>MGSSHHHHHHHHHHSSGLVPRGSGGSMSAIGTVFKEHVKNFYLIQRLAQFQVKIINHSNYLGVAWELINPVMQIMVYWMVFGLGIRSNAPIHGVPFVYWLLVGISMWFFINQGILEGTKAITQKFNQVSKMNFPLSIIPTYIVTSRFYGHLGLLLLVIIACMFTGIYPSIHIIQLLIYVPFCFFLTASVTLLTSTLGVLVRDTQMLMQAILRILFYFSPILWLPKNHGISGLIHEMMKYNPVYFIAESYRAAILYHEWYFMDHWKLMLYNFGIVAIFFAIGAYLHMKYRDQFADFL[2x];>MNVSVNIKNVTKEYRIYRTNKERMKDALIPKHKNKTFFALDDISLKAYEGDVIGLVGINGSGKSTLSNIIGGSLSPTVGKVDRNGEVSVIAISAGLSGQLTGIENIEFKMLCMGFKRKEIKAMTPKIIEFSELGEFIYQPVKKYSSGMRAKLGFSINITVNPDILVIDEALSVGDQTFAQKCLDKIYEFKEQNKTIFFVSHNLGQVRQFCTKIAWIEGGKLKDYGELDDVLPKYEAFLNDFKKKSKAEQKEFRNKLDESRFVIK[2x]

Wall teichoic acid (WTA) is a polyol phosphate polymer that covalently decorates peptidoglycan of gram-positive bacteria, including Staphylococcus aureus. Central to WTA biosynthesis is flipping of lipid-linked precursors across the cell membrane by TarGH, a type V ABC transporter. TarGH is a heterotetramer composed of two TarG polytopic transmembrane domains (TMD) and two TarH nucleotide binding domains (NBD). Like other ABC transporters, TarGH uses the energy derived from the ATP hydrolysis cycle in the NBDs to drive substrate transport across the membrane via the TMDs.

The cryo-EM structure of S. aureus TarGH in complex with ATPγS was determined to 2.3 Å resolution. One of the highest resolution ABC transporters yet determined by cryo-EM, the quality of the reconstruction permitted confident modelling of the complete sequences of TarG and TarH. In this ATPγS-bound state, three well-ordered LMNG molecules are observed. Two are bound in symmetrically disposed wedge-shaped clefts formed at the inner leaflet/cytosol interface between the TarH GH, TarG IFc and the LG-loop on the opposing TarG protomer (denoted LMNGC). The third ordered LMNG is observed on the extracellular face of TarG, on the dimer rotation axis (LMNGE). The level of detail at 2.3 Å resolution allowed unambiguous modelling of key active site features that show it to be in a non-optimal configuration for ATP hydrolysis. The aliphatic side chain of Val173 is inserted into a hydrophobic pocket, which includes invariant aromatics Phe154 and Phe178, with its backbone carbonyl flipped away from the active site and no longer in position to coordinate the catalytic water during ATP hydrolysis (we designate this D-loopOFF). An additional consequence of this rearranged D-loopOFF is the creation of a solvent exposed cytoplasmic channel of ~10 Å across at its narrowest that runs through the NBD dimer, continuous with the electropositive intramembrane cavity between the two TarG protomers. We speculate therefore that the LMNGC-bound (D-loopOFF) structure represents a substrate loaded state with the cytoplasmically oriented lipid-linked polymer captured at the inner leaflet of the membrane but prior to polymer insertion and translocation.>GTSSMADIGSRYSKISDNYSSLLQVSEALGRAGLESSNLIVGIDFTKSNEWTGAKSFNRKSLHHLSNTPNPYEQAITIIGRTLAAFDEDNLIPCYGFGDASTHDQDVFSFYPEGRFCNGFEEVLARYREIVPQLKLAGPT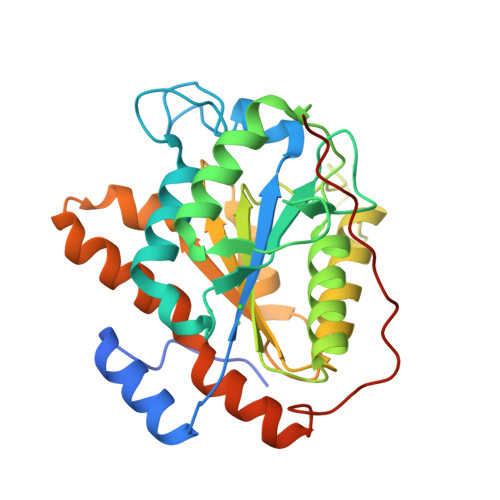SFAPIIEMAMTVVEQSSGQYHVLVIIADGQVTRSVDTEHGRLSPQEQKTVDAIVKASTLPLSIVLVGVGDGPWDMMQEFDDNIPARAFDNFQFVNFTEIMSKNKDQSRKETEFALSALMEIPPQYKATIELNLLGVRNGNIPQRIPLPPPVQSGSSFSSSR[2x]> PLGSMPFH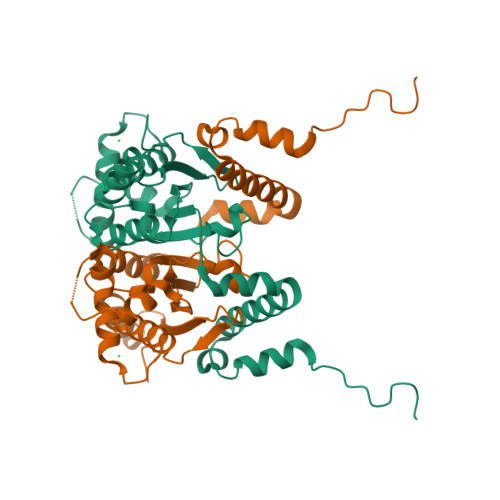AEPLKPSDEIDMDLGHSVAAQKFKEIREVLEGNRYWARKVTSEEPEFMAEQVKGQAPNFLWIGCADSRVPEVTIMARKPGDVFVQRNVANQFKPEDDSSQALLNYAIMNVGVTHVMVVGHTGCGGCIAAFDQPLPTEENPGGTPLVRYLEPIIRLKHSLPEGSDVNDLIKENVKMAVKNVVNSPTIQGAWEQARKGEFREVFVHGWLYDLSTGNIVDLNVTQGPHPFVDDRVPRA> GDRVADVIESSIGDSV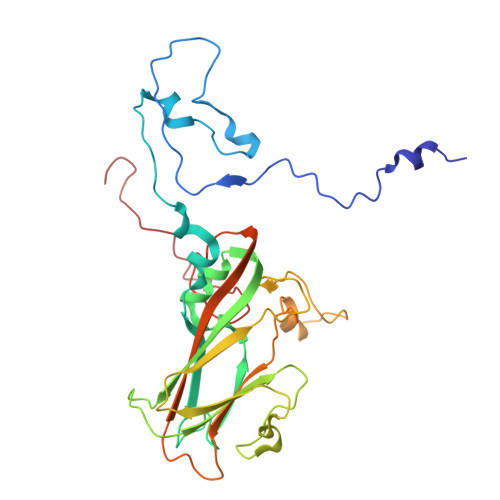SRALTQALPAPTGQNTQVSSHRLDTGEVPALQAAEIGASSNTSDESMIETRCVLNSHSTAETTLDSFFSRAGLVGEIDLPLEGTTNPNGYANWDIDITGYAQMRRKVELFTYMRFDAEFTFVACTPTGQVVPQLLQYMFVPPGAPKPESRESLAWQTATNPSVFVKLTDPPAQVSVPFMSPASAYQWFYDGYPTFGEHKQEKDLEYGACPNNMMGTFSVRNVGSSKSKYPLVVRIYMRMKHVRAWIPRPMRNQNYLFKANPNYAGNSIKPTGTSRTAITTL>[2x]PRILGRNIGSHHVRVEHFMNH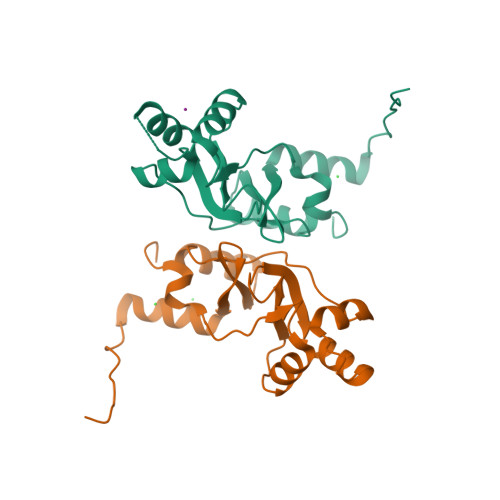SITTLAKDTPLEEVVKVVTSTDVTEYPLVESTESQILVGIVQRAQLVQALQAEPPSRAPGHQQCLQDILARGCPTEPVTLTLFSETTLHQAQNLFKLLNLQSLFVTSRGRAVGCVSWVEMKKAISNLTNPPAPKEFLEVLFQG2-fluoranyl-5-[2-[(4~{R})-4-methyl-2-oxidanylidene-4-phenyl-pyrrolidin-1-yl]ethoxy]benzenecarbonitrile 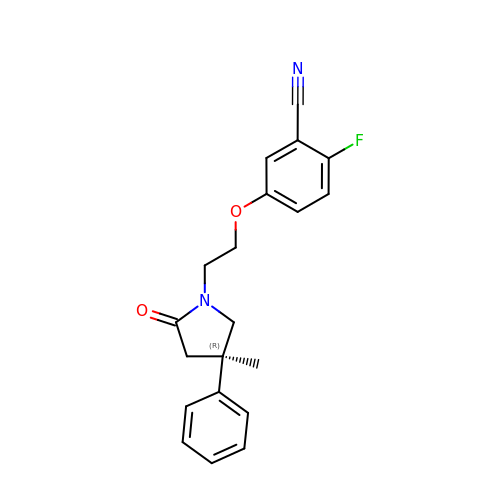| C20 H19 F N2 O2 | WMVNTKWNIVSPIC-FQEVSTJZSA-N> SMATSNLLKNKGSLQFEDKWDFMRPIVLKLLRQESVTKQQWFDLFSDVHAVCLWDDKGPAKIHQALKEDILEFIKQAQARVLSHQDDTALLKAYIVEWRKFFTQCDILPKPFCQLEITLMGKQGSNKKSNVEDSIVRKLMLDTWNESIFSNIKNRLQDSAMKLVHAERLGEAFDSQLVIGVRESYVNLCSNPEDKLQIYRDNFEKAYLDSTERFYRTQAPSYLQQNGVQNYMKYADAKLKEEEKRALRYLETRRECNSVEALMECCVNALVTSFKETILAECQGMIKRNETEKLHLMFSLMDKVPNGIEPMLKDLEEHIISAGLADMVAAAETIT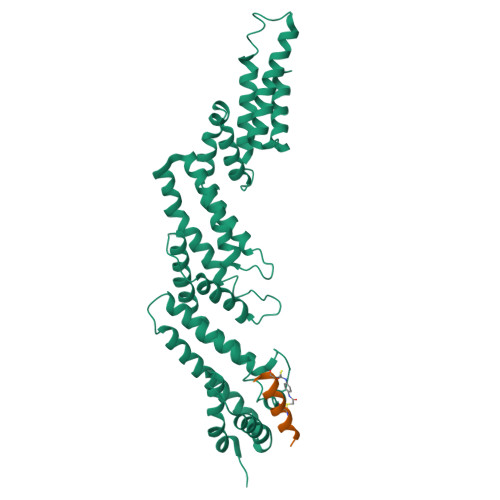TDSEKYREQLDTLFNRFSKLVKEAFQDDPRFLTARDKAYKAVVNDATIFKLE;> XDPAWYDCADAAWICTFX> SKGLEDSSTISFITWNIDGLDGCNLPERARGVCSCLALYSPDVVFLQEVIPPYCAYLKKRAASYTIITGNEEGYFTAILLKKGRVKFKSQEIIPFPNTKMMRNLLCVNVSLGGNEFCLMTSHLESTREHSAERIRQLKTVLGKMQEAPDSTTVIFAGDTNLRDQEVIKCGGLPDNVFDAWEFLGKPKHCQYTWDTKANNNLRIPAAYKHRFDRIFFRAEEGHLIPQSLDLVGLEKLDCGRFPSDHWGLLCTLNVVL;> SN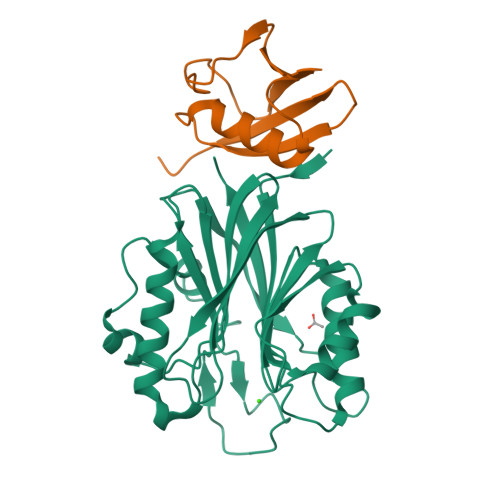VKTENNDHINLKVAGQDGSVVQFKIKRHTPLSKLMKAYCERQGLSMRQIRFRFDGQPINETDTPAQLEMEDEDTIDVFQQQTGG High expression of PSMαs, which are four peptides of about 20-residues in length, increases virulence potential of methicillin-resistant S. aureus (MRSA). Amyloid aggregation plays roles in PSM activities in S. aureus. In the present study, we investigated the structure-function relationships of PSMαs and their short truncations.

We found that the LFKFFK segment from PSMα3, identified as fibril-forming by computational methods and which indeed forms fibrils, shows dose-dependent antibacterial activity against Gram-positive Micrococcus luteus and Staphylococcus hominis, but is nontoxic to S. aureus, the secreting bacterium. We obtained two atomic resolution structures of LFKFFK; both revealed a departure from cross-β fibrils and atypical amyloid architectures. The second polymorph was composed of out-of-register β-sheets, meaning that unlike in canonical cross-β fibrils, β-strands are not perpendicular to the fibril axis. The second polymorph, featuring out-of-register β-sheets, shows intermediate quantitative measures of amyloid stability, consistent with the previous suggestion that this mating configuration could be associated to the transient nature of amyloid oligomers. The second polymorph of LFKFFK is composed of out-of-register β-sheets, a morphology that was also suggested to serve as a pathway to toxic amyloid aggregates, and the interface between the sheets is reminiscent of the KLVFFA segment of amyloid-β42. Thus, the two different polymorphs of the antibacterial peptide LFKFFK display features which, in human disease-associated amyloids, correlate with toxicity. We correspondingly suggest that atypical fibrils of LFKFFK encode toxicity to bacteria, while the reversible fibril formation provides means to regulate activity. By not representing a spine that recapitulates the properties of the full-length PSMα3, the LFKFFK segment exemplifies how an array of activities can be derived from a single polypeptide, through generation of shorter derivatives with different structural properties.

>LFKFFK[2x]>MFKKLLDNKNLVINPPVFITSILLIVALILTCVLFPEKVGVWFPAAQLAVTSNFGWFFVVTVNVILIFAIYLAFSKFGRIRLGGDDAEPEFTKASWFAMLFSTGMGIGIMFFSIAEPVSHFFNTPRPVDTDIEAAVQAMQFTSLHWGLHAWGIYAMVGLALAFFGFNRKLPMTFRSLFYPFWGERIHGWWGHIIDILSALATVFGLSTSLGLGVIQITAGLEYLYGWEISPMMQAGIILFVIGIATISVFSGLDKGVKILSNANMYIAASFMLLIFILGPTLFIMKGYVENTGAYLANFIDISTWNDTYLGSGWQNVWTIFYWAWWIAWSPFVGSFIARISKGRTVKEFVLGVLIVPGLITLLWMNVFGGSALHTILSGDVTMIAAVKADVSTALFVFLENFPFTKFLSIVAIILIFSFFITSSDSGSLVVDNITSGSNGESPVWQRVFWSFAQGIIAIVLLWGGGLDALQTAVIITGLPFAVILLVMCYSLQKGLKEELAKSSKKAKSKEEKSYKEIIAELLDEPQSKHHHHHHHHHH[3x]

Thus, in the deep-sea bacterium Myroides profundi D25, TMA is taken into the cells through a TMA transporter TmaT and then oxidized to TMAO, resulting in the accumulation of intracellular TMAO to millimolar levels to function as a piezolyte. TmaT is a member of the betaine-choline-carnitine transporter family, and we show that TmaT is an Na+/TMA symporter, which possessed high specificity and binding affinity toward TMA. TmaT forms a homotrimer structure in solution. Each TmaT monomer has 12 transmembrane helices, and the TMA transport channel is formed by a four-helix bundle.

To elucidate the mechanism of TmaT importing TMA, we employed the cryo-EM single-particle technique to determine the TmaT structure. TmaT assembles a homotrimer in solution, similar to other reported structures of BCCT carriers. The overall structure of TmaT consists of three regions: the extracellular, intracellular, and transmembrane regions, with the overall transmembrane width of approximately 33 Å. The structures of the three TmaT monomers are nearly identical (with the root mean square deviation [RMSD] of 0.2–0.4 Å), with each monomer forms a cylindrical structure consisting of 12 transmembrane helices (TM1–TM12). Most of the transmembrane helices are connected by short loops, with the exception for TM7 and TM8, which are linked by a long helix (H7). TM3 and TM8 consist of both inner membrane portions (TM3i and TM8i) and outer membrane portions (TM3e and TM8e), making them discontinuous transmembrane helices. In the TmaT trimer structure, the loop Thr304-Gly313 from one monomer inserts into an adjacent monomer and resembles a gate latch and bolt pattern. In addition, hydrogen bond interactions are formed with the residues Glu290, Asn291, Thr308, and Tyr309 in the interface between two adjacent monomers, suggesting a relatively stable trimer composition. Comparison of the TmaT and TmaT-TMA LCI structures revealed that the side chain of Met105 occupies the TMA-binding site when TMA is not bounded, suggesting an important role of Met105 in TMA recognition. However, they diverge in substrate recognition, as the side chain of Met105 in TmaT occupies the substrate-binding pockets during substrate binding, a characteristic not observed in the structures of BetP and CaiT.>[2x]GSPNSGTLALLLDEGSKQLPQAIIIGVKKGGTRALLEFLRVHPDVRAVGAEPHFFDRSYDKGLAWYRDLMPRTLDGQITMEKTPSYFVTREAPARISAMSKDTKLIVVVRDPVTRAISDYTQTLSKRPDIPTFESLTFKNRTAGLIDTSWSAIQIGIYAKHLEHWLRHFPIRQMLFVSGERLISDPAGELGRVQDFLGLKRIITDKHFYFNKTKGFPCLKKAEGSSRPHCLGKTKGRTHPEIDREVVRRLREFYRPFNLKFYQMTGHDFGWDG

Heparan sulfate 3-O-sulfotransferase (3-OST), the enzyme responsible for completing this modification, is present in seven different isoforms in humans. The enzymes transfer a sulfo group to the 3-OH position of glucosamine in HS. Individual isoforms display substrate selectivity to uniquely sulfated saccharide sequences present in heparan sulfate polysaccharides. Here, we report two ternary crystal structures of heparan sulfate 3-OST isoform 3 (3-OST-3) with PAP (3′-phosphoadenosine 5′-phosphate) and two octasaccharide substrates: non 6-O-sulfated octasaccharide (8-mer 1) and 6-O-sulfated octasaccharide (8-mer 3).

We also obtained the crystal structure of 3-OST-3 bound to PAP and 8-mer 3 at 1.55 Å (ESI†). The complex was crystallized in a different space group but with a similar asymmetric unit dimer of 3-OST-3 containing PAP and an 8-mer 3 substrate. Despite the presence of 6-O-sulfo groups, this substrate superimposes well with the 8-mer 1 substrate, positioning the acceptor in the same position with respect to PAP. Notably, the presence of the 6-O-sulfo groups generate additional potential hydrogen interactions between 3-OST-3 and saccharides a, c, and e (ESI†). These additional interactions may account for the apparent increase in binding affinity of 8-mer 3 versus 8-mer 1. Surprisingly, the 8-mer 3 binds to the other molecule in the asymmetric unit in a completely different orientation (ESI†). A superposition of the two 3-OST-3 molecules within the asymmetric unit (RMSD 0.48 Å on 252 Cα atoms) reveals the other 8-mer 3 is binding across the cleft in the opposite direction from that of the previous oligosaccharide. The 8-mer 3 is offset such that the uronic acids, GlcA (saccharide h) and IdoA2S (saccharide f), now lie in the GlcNS6S saccharide c and e sites, and the acceptor GlcNS6S (saccharide e) is positioned with its 3-OH distal from the active site. However, it is located 7.4 Å away from the phosphorus atom of the 5′ phosphate and not in-line. This binding orientation is likely inconsistent with transfer of the sulfo group to the acceptor site, thereby, it is deemed to represent non-productive binding. A kink in 8-mer 3 is visible due to IdoA2S (saccharide f) being in the 1C4 conformation, as opposed to the 2SO observed in the productive orientation (ESI†).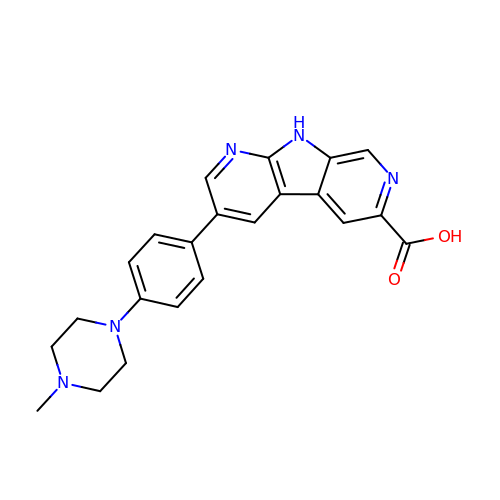3-[4-(4-methylpiperazin-1-yl)phenyl]-9H-pyrrolo[2,3-b:5,4-c']dipyridine-6-carboxylic acid | C22 H21 N5 O2 | AVGXCPYDUVBUKP-UHFFFAOYSA-N>GSGSGMDEIVKVLSQHDRILVVGHIMPDGDCVSSVLSLTLGLEKLGKEVKAAVDYKIPYVFEKFPYIDKIEENPNFDPELLVVVDASSPDRIGKFQDLLDKVPSVVIDHHSTNTNFGNWNWVDPSFAATAQMIFRINKALGVEYDSNLATLNYLGIATDTGFFRH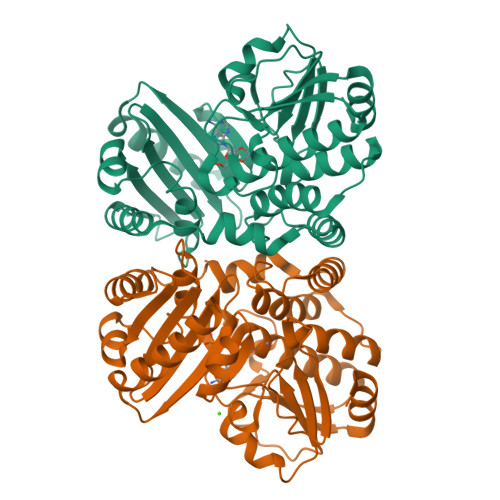SNADVRVFEDAYKLVKMGADAHFVAKEILENKRFEQFKLFAEVLERLQLLENGKIAYSYIDYDTYLRHNCTDEDSAGFVGELRSIRGVEVAVLFMEFPRGKIHVSMRSKDWFNVNEVAFELGGGGHPRAAGVTFEGKKIEEVIPRVINHLLKKFKEGVESESEKIPEGDVLGG[2x]5-FLUORO-9-AMINO-(N-(2-DIMETHYLAMINO)ETHYL)ACRIDINE-4-CARBOXAMIDE | C18 H19 F N4 O | 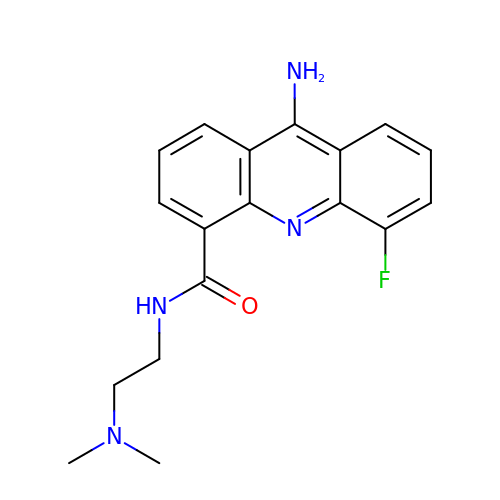QEHXKZSBSOBCGM-UHFFFAOYSA-N> GVGISTGTFNNQTEFKFLENGWVEITANSSRLVHLNMPESENYRRVVVNNMDKTAVRGNMALDDIHAQIVTPWSLVDANAWGVWFNPGDWQLIVNTMSELHLVSFEQEIFNVVLKTVSESATQPPTKVYNNDLTASLMVALDSNNTMPFTPAAMRSETLGFYPWKPTIPTPWRYYFQWDRTLIPSHTGTSGTPTNIYHGTDPDDVQFYTIENSVPVHLLRTGDEFATGTFFFDCKPCRLTHTWQTNRALGLPPFLNSLPQSEGATNFGDIGVQQDKRRGVTQMGNTNYITEATIMRPAEVGYSAPYYSFEASTQGPFKTPIAAGRGGAQTDENQAADGNPRYAFGRQHGQKTTTTGETPERFTYIAHQDTGRYPEGDWIQNINFNLPVTNDNVLLPTDPIGGKTGINYTNIFNTYGPLTALNNVPPVYPNGQIWDK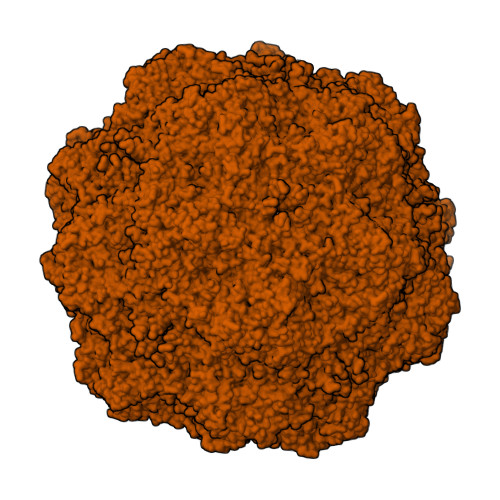EFDTDLKPRLHVNAPFVCQNNCPGQLFVKVAPNLTNEYDPDASANMSRIVTYSDFWWKGKLVFKAKLRASHTWNPIQQMSINVDNQFNYVPSNIGGMKIVYEKSQLAPRKLY>MTKNVADELAGLELPVERGCPFAPPAAYERLRERAPINKVRLTSGGQAWWVSGHEEARAVLADGRFSSDKRKDGFPLFTLDAATLQQLRSQPPLMLGMDGAEHSAARRPVIGEFTVKRLAALRPRIQDIVDHFIDDMLATDQRPVDLVQALSLPVPSLVICELLGVPYTDHDFFQSRTTMMVSRTSMEDRRRAFAELRAYIDDLITRKESEPGDDLFSRQIARQRQEGTLDHAGLVSLAFLLLTAGHETTANMISLGVVGLLSHPEQLTVVKANPGRTPMAVEELLRYFTIADGVTSRLATEDVEIGGVSIKAGEGVIVSMLSA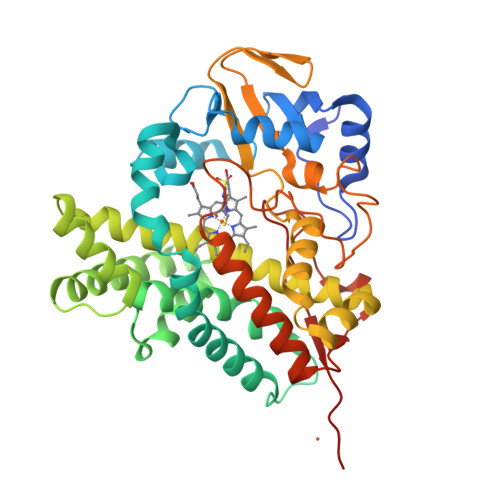NWDPAVFKDPAVLDVERGARHHLAFGFGPHQCLGQNLARMELQIVFDTLFRRIPSLRLAVPMEDVPFKGDSVIYGVHELPVTWHHHHHH[2x]2-METHYL-FURAN-3-CARBOTHIOIC ACID 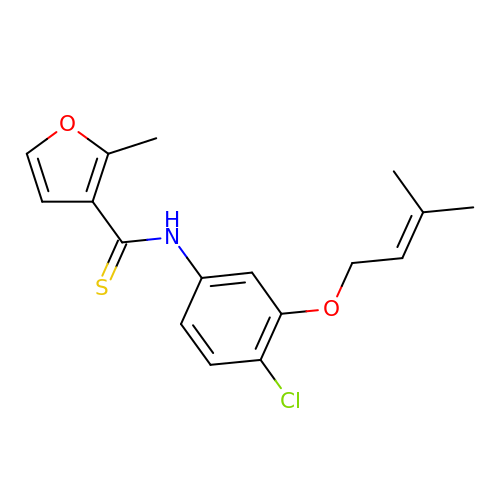[4-CHLORO-3-(3-METHYL-BUT-2-ENYLOXY)-PHENYL]-AMIDE | C17 H18 Cl N O2 S | YZHIXLCGPOTQNB-UHFFFAOYSA-N> MSKGASAPQQQSAFKQLYTELFNNEGDFSKVSSNLKKPLKCYVKESYPHFLVTDGYFFVAPYFTKEAVNEFHAKFPNVNIVDLTDKVIVINNWSLELRRVNSAEVFTSYANLEARLIVHSFKPNLQERLNPTRYPVNLFRDDEFKTTI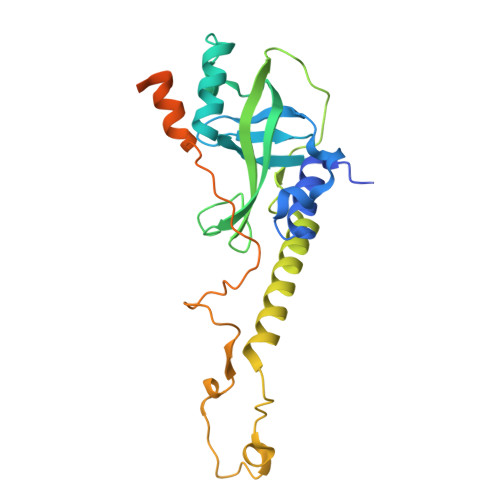QHFRHTALQAAINKTVKGDNLVDISKVADAAGKKGKVDAGIVKASASKGDEFSDFSFKEGNTATLKIADIFVQEKGKDALNKAADHTDGAKVKGGAKGKGKAAAKAAKGKKL>GAEAGITGTWYNQSGSTFTVTAGADGNLTGQYENRAQGTGCQNSPYTLTGRYNGTKLEWRVEWNNSTENCHSRTEWRGQYQGGAEARINT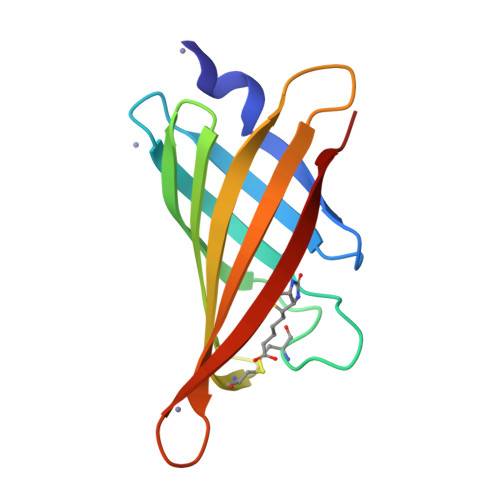QWNLTYEGGSGPATEQGQDTFTKVK[4x]HEXYLPHOSPHONIC ACID (S)-2-METHYL-3-PHENYLPROPYL ESTER 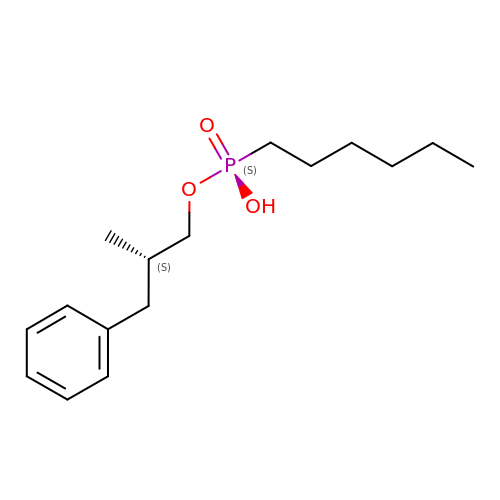| C16 H27 O3 P | MMTDYBZZRYOMFD-HNNXBMFYSA-N ethyl (9~{R})-2-methoxy-4-oxidanylidene-9-[[(1~{S})-1-phenylethyl]-[(2-propan-2-ylphenyl)carbamoyl]amino]-6,7,8,9-tetrahydropyrido[1,2-a]pyrimidine-3-carboxylate | C30 H36 N4 O5 | 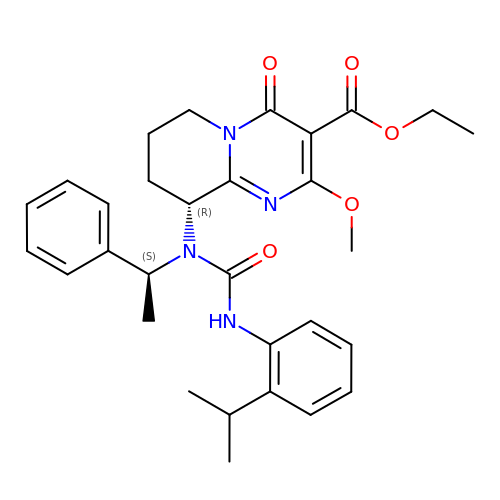MLCVKHFILIDRCO-UHFFFAOYSA-N> FDVGDEYEIIETIGNGAYGVVSSARRRLTGQQVAIKKIPNAFDVVTNAKRTLRELKILKHFKHDNIIAIKDILRPTVPYGEFKSVYVVLDLMESDLHQIIHSSQPLTLEHVRYFLYQLLRGLKYMHSAQVIHRDLKPSNLLVNENCELKIGDFGMARGLCTSPAEHQYFMTEYVATRWYRAPELMLSLHEYTQAIDLWSVGCIFGEMLARRQLFPGKNYVHQLQLIMMVLGTPSPAVIQAVGAERVRAYIQSLPPRQPVPWETVYPGADRQALSLLGRMLRFEPSARISAAAALRHPFLAKYHDPDDEPDCAPPFDFAFDREALTRERIKEAIVAEIEDFHARREG

The ERK5 protein, which is encoded by the MAPK7 gene, comprises an N-terminal kinase domain and a large C-terminal domain containing transcriptional transactivating functionality and nuclear localization and export sequences (NLS/NES). ERK5 is the effector kinase of a canonical kinase module comprising MEK (MAPK/ERK kinase) 5, MEKK (MEK kinase) 2/3 and ERK5 itself.

Compound 2 has a primary alcohol in place of the methylpiperazine group of compound 1, an N-methyl in place of the N-cyclopentyl substituent on the tricyclic ring system, and an O-ethyl in place of an O-methyl at the meta-position of the phenyl group. These changes combine to yield a compound with a similar inhibitory potency to compound 1. The conventional, so-called type I, kinase inhibitor-binding mode is demonstrated by structures of ERK5 co-crystallized with the aminopyrimidine-containing compounds 2 and 3, while a novel allosteric binding mode was observed for three triazole-containing compounds (compounds 4–6). Compounds 2 and 3, like compound 1, bind at the conventional ATP-binding site, while compounds 4, 5 and 6 bind at a novel allosteric binding site. The aminopyrimidine motif forms a hydrogen-bond network with the backbone of Met140 in the ERK5 hinge region. The tricyclic ring systems of compound 1, and to a somewhat lesser extent compound 2, however, occupy a greater volume than the equivalent region of compound 3, with the benzene-ring fragment extending downwards to fit into the base of the ATP-binding site, whilst in compound 1 the N-cyclopentyl substituent points upwards towards the P-loop and packs against Ile61. Residues 208–215, corresponding to the central portion of the activation loop, could not be modelled in the complex with compound 2. As observed for the complex of compound 1 with ERK5, compounds 2–5 bind to a ‘DFG-in’ conformation of ERK5 in which both the hydrophobic R-spine (residues Leu106, Ile117, His180 and Phe201 in ERK5) and C-spine (Val69, Ala82, Leu144, Leu188, Leu189, Val190, Ile251 and Met255) are intact. Compounds 2, 3 and 5 were tested against a panel of 225 kinases representative of the kinome to assess the selectivity of these three different scaffolds. The kinase selectivity-profile data show that compound 5 is the most selective, while compound 3 is the most promiscuous, with the selectivity of compound 2 being intermediate.>MSFSQAVSGLNAAATNLDVIGNNIANSATYGFKSGTASFADMFAGSKVGLGVKVAGITQDFTDGTTTNTGRGLDVAISQNGFFRLVDSNGSVFYSRNGQFKLDENRNLVNMQGMQLTGYPATGTPPTIQQGANPAPITIPNTLMAAKSTTTASMQINLNSTDPVPSKTPFSVSDADSYNKKGTVTVYDSQGNAHDMNVYFVKTKDNEWAVYTHDSSDPAATAPTTASTTLKFNENGILESGGTVNITTGTINGATAATFSLSFLNSMQQNTGANNIVATNQNGYKPGDLVSYQINNDGTVVGNYSNEQEQVLGQIVLANFANNEGLASQGDNVWAATQASGVALLGTAGSGNFGKLTNGALEASNVDLSKELVNMIVAQRNYQSNAQTIKTQDQILNTLVNLR[13x];>[11x]MSSLINHAMSGLNAAQAALNTVSNNINNYNVAGYTRQTTILAQANSTLGAGGWIGNGVYVSGVQREYDAFITNQLRGAQNQSSGLTTRYEQMSKIDNLLADKSSSLSGSLQSFFTSLQTLVSNAEDPAARQALIGKAEGLVNQFKTTDQYLRDQDKQVNIAIGSSVAQINNYAKQIANLNDQISRMTGVGAGASPNDLLDQRDQLVSELNKIVGVEVSVQDGGTYNLTMANGYTLVQGSTARQLAAVPSSADPTRTTVAYVDEAAGNIEIPEKLLNTGSLGGLLTFRSQDLDQTRNTLGQLALAFADAFNAQHTKGYDADGNKGKDFFSIGSPVVYSNSNNADKTVSLTAKVVDSTKVQATDYKIVFDGTDWQVTRTADNTTFTATKDADGKLEIDGLKVTVGTGAQKNDSFLLKPVSNAIVDMNVKVTNEAEIAMASESKLDPDVDTGDSDNRNGQALLDLQNSNVVGGNKTFNDAYATLVSDVGNKTSTLKTSSTTQANVVKQLYKQQQSVSGVNLDEEYGNLQRYQQYYLANAQVLQTANALFDALLNIR;>[11x]MRISTQMMYEQNMSGITNSQAEWMKLGEQMSTGKRVTNPSDDPIAASQAVVLSQAQAQNSQYALARTFATQKVSLEESVLSQVTTAIQTAQEKIVYAGNGTLSDDDRASLATDLQGIRDQLMNLANSTDGNGRYIFAGYKTEAAPFDQATGGYHGGEKSVTQQVDSARTMVIGHTGAQIFNSITSNAVPEPDGSDSEKNLFVMLDTAIAALKTPVEGNNVEKEKAAAAIDKTN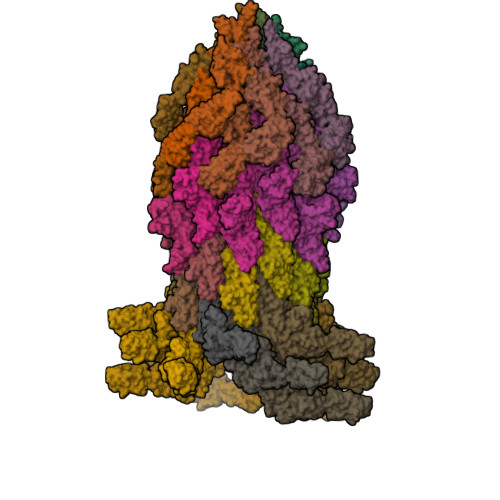RGLKNSLNNVLTVRAELGTQLSELSTLDSLGSDRALGQKLQMSNLVDVDWNSVISSYVMQQAALQASYKTFTDMQGMSLFQLNR;>[15x]MAQVINTNSLSLLTQNNLNKSQSALGTAIERLSSGLRINSAKDDAAGQAIANRFTANIKGLTQASRNANDGISIAQTTEGALNEINNNLQRVRELAVQSANSTNSQSDLDSIQAEITQRLNEIDRVSGQTQFNGVKVLAQDNTLTIQVGANDGETIDIDLKQINSQTLGLDTLNVQQKYKVSDTAATVTGYADTTIALDNSTFKASATGLGGTDQKIDGDLKFDDTTGKYYAKVTVTGGTGKDGYYEVSVDKTNGEVTLAGGATSPLTGGLPATATEDVKNVQVANADLTEAKAALTAAGVTGTASVVKMSYTDNNGKTIDGGLAVKVGDDYYSATQNKDGSISINTTKYTADDGTSKTALNKLGGADGKTEVVSIGGKTYAASKAEGHNFKAQPDLAEAAATTTENPLQKIDAALAQVDTLRSDLGAVQNRFNSAITNLGNTVNNLTSARSRIEDSDYATEVSNMSRAQILQQAGTSVLAQANQVPQNVLSLLR>[2x]AEEWYFGKITRRESERLLLNPENPRGTFLVRESETT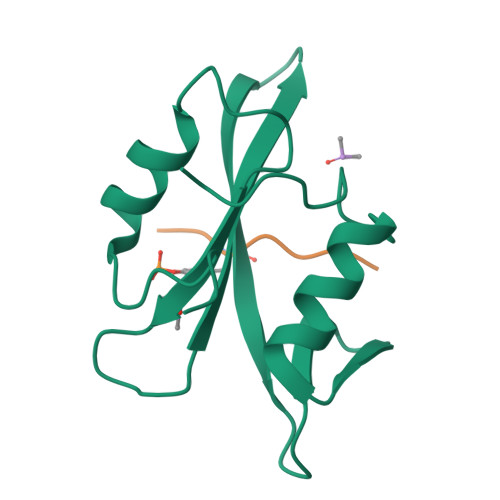KGAYCLSVSDFDNAKGLNVKHYKIRKLDSGGFYITSRTQFSSLQQLVAYYSKHADGLCHRLTNVCP;>CDYANFK[2x]>AVGIFVIIFGIALFFLAMKVSGLVGTNLSDGYTMKAQFDNVNGLKPRAKVTMSGVTIGRVDSITLDPVTRLATVTFDLDGKLTSFNAEQLKEVQKNALDELRYSSDYTQATPAQQKTMEQQLISNMNSITSIDEDAYIMVATNGLLGEKYLKIVPGGGLNYLKRGDTISNTQGTMDLEDLISK[6x];>MNTIAWLGRLVIERIRGIGVAALMLLQIIFSLPSAGGFGRFVYQMHRVGVMSLLIITVSGLFIGLVLGLQGYSILVNVGSESMLGTMVSLTLLRELAPVVAALLFAGRAGSALTAEIGSMKQSEQLASMEMIGVDPLKQIVSPRLWAGIVSLPMLTVIFAAIGIVGGKLVGVDFLGVDEGSFWSGMQNNVQFGHDVVNGIIKSIVFALLCTWIAVFQGYACDPTPEGIATAMTRTVVYSSLCVLGFDFVLTAVMFGG[2x];>[2x]LIEVKNLSFNRGERVIYDNISLNIRRGQITAIMGPSGTGKTTLLRLIGGQLVPDQGEVLLDGKDIAQMSRQRARMGMLFQSGALFTDMSVYENVAFPIRAHTLSENLIAELVALKLESVGLRGTEQLMPTELSGGMNRRVALARAIALDPDLIMYDEPFAGQDPIVKGVLTRLIRSLREALDLTTIIVSHDVPETLSIADYIYVVAEGKIQGEGTPEELQAYASPFVKQFLTG;>VQYLNQELVVSGKIDFENAEQQYQAGLAIIKKQTSFPLIVDLKQLEHGNTLALAVLVQWLRQTPQKSGLHFKNVPEKMLKIIQACHLQEDLHL[2x]

We performed a genetic screen to identify genes important for the OM barrier of A. baumannii. This led to the identification of an ABC (ATP-binding cassette) transporter complex that promotes GPL export to the OM. The A. baumannii operon includes: mlaF and mlaE, respectively predicted to encode the nucleotide-binding and transmembrane domains of an ABC transporter; mlaD, encoding a protein containing an IM-spanning domain and a predicted periplasmic soluble domain; mlaC, encoding a soluble periplasmic protein; and mlaB, an additional gene predicted to encode a cytoplasmic sulfate transporter and anti-sigma factor antiagonist (STAS)-domain protein. The results of the stable isotope pulse experiments in the ∆mlaA strain revealed results consistent with those obtained from ∆mlaC and ∆mlaF, in which the ratio of labeled to unlabeled GPL is consistently higher in the inner membrane than the outer membrane after one hour of exposure to 13C-acetate. These results are consistent with a model in which the IM-localized ABC transporter complex MlaBDEF first transfers GPLs to the periplasmic binding protein MlaC, which then transports GPL to the OM, whereupon MlaA facilitates GPL insertion into the OM. According to this model, ATP hydrolysis by MlaF provides the initial energy to extract GPL from the IM, while the substrate binding components MlaD and MlaC take up lipids for delivery to the OM.

We next used cryo-electron microscopy to characterize the architecture of the A. baumannii MlaBDEF complex (abMlaBDEF). Following 2D- and 3D-classification, we obtained a final dataset of ~14,000 particles with which we obtained a structure to a resolution of 8.7 Å. Based on the bioinformatically-predicted localization of individual proteins and work recently performed on the similar E. coli Mla complex (ecMlaBDEF), we propose that MlaD localizes to the periplasmic side of the IM, MlaE forms the central transmembrane region, and MlaF and MlaB form the bottom layer on the cytoplasmic face of the IM with two visible hetero-dimers. We note that a clear six-fold symmetry is present for the region of the map attributed to MlaD, despite the fact that we only imposed a 2-fold symmetry averaging. We next modeled abMlaD, using an evolution restraints-derived structural model of ecMlaD as a template, and used our previously-published EM-guided symmetry modeling procedure to model its hexameric state. The localization of this extra density suggests that it corresponds to a ~ 45 amino-acid insert present between strands 4 and 5 of the abMlaD β-sheet. Interestingly, the arrangement of MlaF clearly resembles the pre-translocation state of MalK. The resulting MlaE dimer model fits well to the EM map density, and clearly corresponds to a closed transporter, with no solvent channel between the subunits. Interestingly, we also noted clear density for three TM helices that likely correspond to the MlaD N-terminal helices.>[2x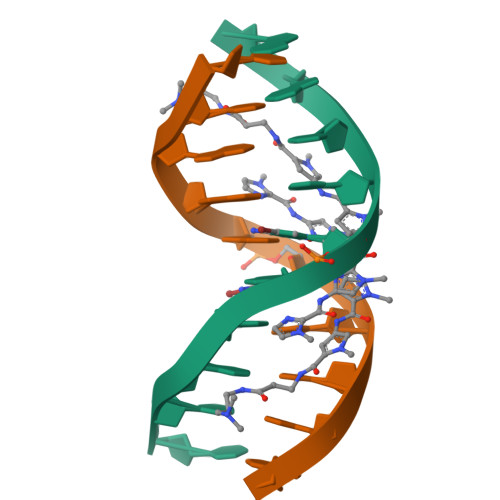]CCAGGCCTGG> MDSLSVNQILYPEVHLDSPIVTNKIVAILEYARVPHAYSLEDPTLCQNIKHRLKNGFSNQMIINNVEVGNVIKSKLRSYPAHSHIPYPNCNQDLFNIEDKESTRKIRELLKKGNSLYSKVSDKVFQCLRDTNSRLGLGSELREDIKEKVINLGVYMHSSQWFEPFLFWFTVKTEMRSVIKSQTHTCHRRRHTPVFFTGSSVELLISRDLVAIISKESQHVYYLTFELVLMYCDVIEGRLMTETAMTIDARYTELLGRVRYMWKLIDGFFPALGNPTYQIVAMLEPLSLAYLQLRDITVELRGAFLNHCFTEIHDVLDQNGFSDEGTYHELIEALDYIFITDDIHLTGEIFSFFRSFGHPRLEAVTAAENVRKYMNQPKVIVYETLMKGHAIFCGIIINGYRDRHGGSWPPLTLPLHAADTIRNAQASGDGLTHEQCVDNWKSFAGVKFGCFMPLSLDSDLTMYLKDKALAALQREWDSVYPKEFLRYDPPKGTGSRRLVDVFLNDSSFDPYDVIMYVVSGAYLHDPEFNLSYSLKEKEIKETGRLFAKMTYKMRACQVIAENLISNGIGKYFKDNGMAKDEHDLTKALHTLAVSGVPKDLKESHRGGPVLKTYSRSPVHTSTRNVRAAKGFIGFPQVIRQDQDTDHPENMEAYETVSAFITTDLKKYCLNWRYETISLFAQRLNEIYGLPSFFQWLHKRLETSVLYVSDPHCPPDLDAHIPLYKVPNDQIFIKYPMGGIEGYCQKLWTISTIPYLYLAAYESGVRIASLVQGDNQTIAVTKRVPSTWPYNLKKREAARVTRDYFVILRQRLHDIGHHLKANETIVSSHFFVYSKGIYYDGLLVSQ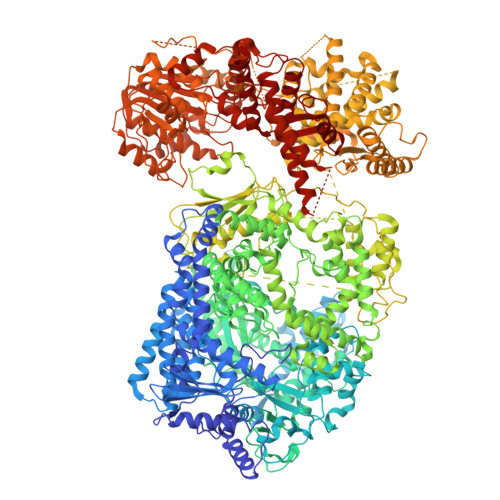SLKSIARCVFWSETIVDETRAACSNIATTMAKSIERGYDRYLAYSLNVLKVIQQILISLGFTINSTMTRDVVIPLLTNNDLLIRMALLPAPIGGMNYLNMSRLFVRNIGDPVTSSIADLKRMILASLMPEETLHQVMTQQPGDSSFLDWASDPYSANLVCVQSITRLLKNITARFVLIHSPNPMLKGLFHDDSKEEDEGLAAFLMDRHIIVPRAAHEILDHSVTGARESIAGMLDTTKGLIRASMRKGGLTSRVITRLSNYDYEQFRAGMVLLTGRKRNVLIDKESCSVQLARALRSHMWARLARGRPIYGLEVPDVLESMRGHLIRRHETCVICECGSVNYGWFFVPSGCQLDDIDKETSSLRVPYIGSTTDERTDMKLAFVRAPSRSLRSAVRIATVYSWAYGDDDSSWNEAWLLARQRANVSLEELRVITPISTSTNLAHRLRDRSTQVKYSGTSLVRVARYTTISNDNLSFVISDKKVDTNFIYQQGMLLGLGVLETLFRLEKDTGSSNTVLHLHVETDCCVIPMIDHPRIPSSRKLELRAELCTNPLIYDNAPLIDRDATRLYTQSHRRHLVEFVTWSTPQLYHILAKSTALSMIDLVTKFEKDHMNEISALIGDDDINSFITEFLLIEPRLFTIYLGQCAAINWAFDVHYHRPSGKYQMGELLSSFLSRMSKGVFKVLVNALSHPKIYKKFWHCGIIEPIHGPSLDAQNLHTTVCNMVYTCYMTYLDLLLNEELEEFTFLLCESDEDVVPDRFDNIQAKHLCVLADLYCQPGTCPPIQGLRPVEKCAVLTDHIKAEAMLSPAGSSWNINPIIVDHYSCSLTYLRRGSIKQIRLRVDPGFIFDALAEVNVSQPKIGSNNISNMSIKAFRPPHDDVAKLLKDINTSKHNLPISGGNLANYEIHAFRRIGLNSSACYKAVEISTLIRRCLEPGEDGLFLGEGSGSMLITYKEILKLSKCFYNSGVSANSRSGQRELAPYPSEVGLVEHRMGVGNIVKVLFNGRPEVTWVGSVDCFNFIVSNIPTSSVGFIHSDIETLPDKDTIEKLEELAAILSMALLLGKIGSILVIKLMPFSGDFVQGFISYVGSHYREVNLVYPRYSNFISTESYLVMTDLKANRLMNPEKIKQQIIESSVRTSPGLIGHILSIKQLSCIQAIVGDAVSRGDINPTLKKLTPIEQVLINCGLAINGPKLCKELIHHDVASGQDGLLNSILILYRELARFKDNQRSQQGMFHAYPVLVSSRQRELISRITRKFWGHILLYSGNRKLINKFIQNLKSGYLILDLHQNIFVKNLSKSEKQIIMTGGLKREWVFKVTVKETKEWYKLVGYSALIKD The replication of positive-strand RNA viruses relies on virally encoded RNA-dependent RNA polymerases (RdRPs) that are capable of rapid and processive synthesis of the 7–14 kilobase viral genomes. To examine this in further detail and to validate the polymerase–RNA interactions seen in the initial poliovirus EC structures, we here present nine new coxsackievirus, rhinovirus, and poliovirus elongation complex structures at resolutions ranging from 2.1 to 2.9 Å. All the complexes feature an upstream RNA duplex that is pinched between the pinky finger and thumb domains such that the RNA exit channel is opened by ≈4 Å as compared to the polymerase alone structures. All of the complexes show the open conformation for the active site wherein the β-strands of motifs A and C are not hydrogen bonded together to fully form the RMM-fold that is commonly utilized by polymerase active sites.

Last, we further extended the length of the RNA duplex to 30 base pairs with a longer (GA)3 locking sequence in the r5 RNA and were able to obtain a third structure of the PV polymerase EC at 2.9 Å resolution (PV_r5). The original junction in the PV_r5 lattice is interesting because while there is density for the nucleic acid phosphate backbone, the bases themselves are only weakly ordered and appear to be loosely associated in multiple conformations. We thus consider this junction to be “sticky” without being highly structured, and it is this stickiness that presumably allows it to accommodate both translation and rotation of the polymerases into a new relative arrangement without destroying the crystal lattice altogether. In fact, the PV_r5 structures shows the downstream template RNA helix rotated by ≈180° such that the 5′ end of the non-template strand sits atop the fingers/thumb domain junction, but again there appear to be no well-defined interactions locking the RNA into this alternate orientation. Consistent with this, the set of PV_r5 structures show the downstream helix rotated by ≈180° such that the 5′ end of the helix is closer to the thumb domain than the fingers domain, but again there are no specific polymerase-RNA interactions that lock the nucleic acid into this particular orientation. However, the PV_r5 and CV_r2 crystal forms continue to diffract and the resulting structures show they accommodate translocation in two different ways that further illustrate the utility and flexibility of the engineered coaxial stacking interactions as a crystallization tool.

>GEIQWMRPSKEVGYPIINAPSKTKLEPSAFHYVFEGVKEPAVLTKNDPRLKTDFEEAIFSKYVGNKITEVDEYMKEAVDHYAGQLMSLDINTEQMCLEDAMYGTDGLEALDLSTSAGYPYVAMGKKKRDILNKQTRDTKEMQKLLDTYGINLPLVTYVKDELRSKTKVEQGKSRLIEASSLNDSVAMRMAFGNLYAAFHKNPGVITGSAVGCDPDLFWSKIPVLMEEKLFAFDYTGYDASLSPAWFEALKMVLEKIGFGDRVDYIDYLNHSHHLYKNKTYCVKGGMPSGMSGTSIFNSMINNLIIRTLLLKTYKGIDLDHLKMIAYGDDVIASYPHEVDASLLAQSGKDYGLTMTPADKSATFETVTWENVTFLKRFFRADEKYPFLIHPVMPMKEIHESIRWTKDPRNTQDHVRSLCLLAWHNGEEEYNKFLAKIRSVPIGRALDLPEYSTLYRRWLDSFGSSSHHHHHH[2x]9-DEAZAGUANINE | C6 H6 N4 O | 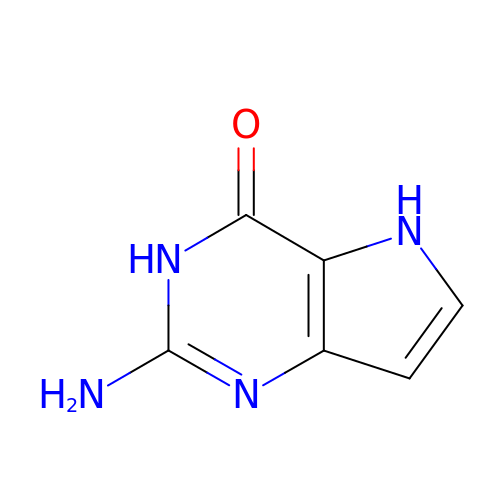FFYPRJYSJODFFD-UHFFFAOYSA-N> ETGPIPMAVVRRELSCESYPIELRCPGTDVIMIESANYGRTDDKICDSDPAQMENIRCYLPDAYKIMSQRCNNRTQCAVVAGPDVFPDPCPGTYKYLEVQYECVPYKVEQKVFLCPGLLKGVYQSEHLFESDHQSGAWCKDPLQASDKIYYMPWTPYRTDTLTEYSSKDDFIAGRPTTTYKLPHRVDGTGFVVYDGALFFNKERTRNIVKFDLRTRIKSGEAIIAN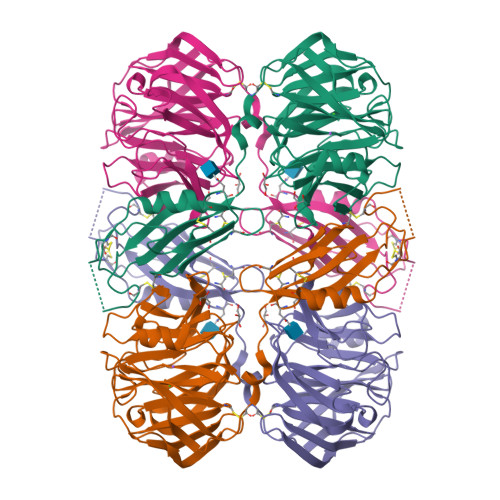ANYHDTSPYRWGGKSDIDLAVDENGLWVIYATEQNNGKIVISQLNPYTLRIEGTWDTAYDKRSASNAFMICGILYVVKSVYEDDDNEATGNKIDYIYNTDQSKDSLVDVPFPNSYQYIAAVDYNPRDNLLYVWNNYHVVKYSLDFGPLDGTKHHHHHH>[2x]GSTYVQALFDFDPQEDGELGFRRGDFIHVMDNSDPNWWKGACHGQTGMFPRNYVTPVNRNV;> GSHMPKMEVFQEYYGIPPPPGAFGPFLRLNPGDIVE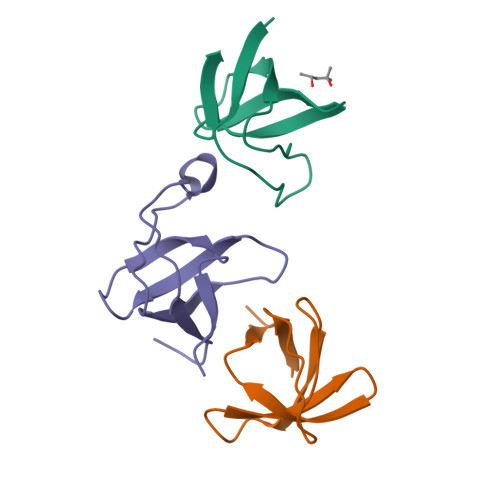LTKAEAEHNWWEGRNTATNEVGWFPCNRVHPYVH> MRIATSPTRRGKNSSVLPLLRRFSWGNGMCSPYYTEHRRQSTLTSSALSSPANHNQQVVYRSIRDCRERAFHLIQELVSSPIPGCGLSYSTNGSFGGPSLTANAVSGVASLLELYDKAYYFL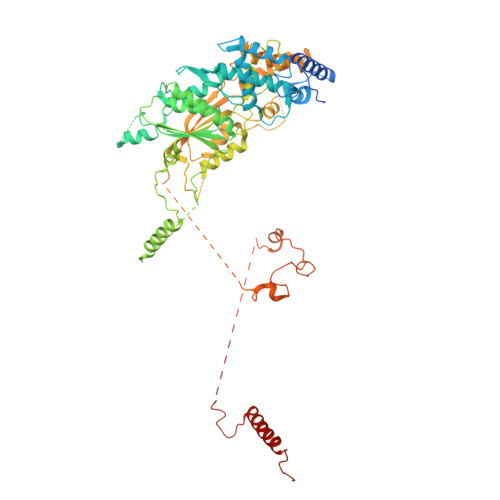HLLHRTILVPRNVVRDTDDFTEFLLRCFRRPSDSLLKGDEELQLSDAAIVDGFVEWMETSLMSAGQFVSFVEVLQLVGSYVRYHKGVRWGARPSEEEWYRCGYRLHPWHDTYCPSSRAEQMPYVHLLQWLMRAKPTKLEEKIDNKEGAHGASSLFSTAAKESAMRAWYATEEFSPPSWHTVVGNSNRLGFTALDCGCHSGYMTELLLKAGAQEVLGVDVSPHHLGNAEATLSEHLRERRSSSHSRKTVQFVRCDILPDLSDEARQTKTPPLGPEGSTNSAAAENRRRLARCHHMPSDSDGLKTETEVTGPFDLLLFHPPLPLLFPTWPLFHDLYESVDQLAYDAGRRHPHCRLSVLNEFLQRLLGSSNGEENNSERRRNAHQQLKHQRRLVAPLIKDNGYVAFILPRNFDTRAILQRMSTSSAGKNCTSCGSDGLAPLVPLSDVVTMTLEGSYTLVLKRSHSLSSLLNRMDYIQKSISAFIRAFVSPQHRSRVEQEVRDFYSNHQAIDLIVMRKIARQKTNEDNNNKDCSVRAVLQKVSEPIAYEDSFEYEEYIPAGGSPLAHHWTEMTPSFSYLEDEFFGCADSVGTNGPPNGASFLAVGHPLVPVTRQLVGVDRFGAGGRDATQGESGNFDKMFAKEMRRRGGRMRKMALTPLEKQEWYIDEKLVKSEAAKVDLMNELSRFELKDFD4-[(1R)-1-aminopropyl]-6-methoxy-2-{6-[4-(propan-2-yl)-4H-1,2,4-triazol-3-yl]pyridin-2-yl}-2,3-dihydro-1H-isoindol-1-one 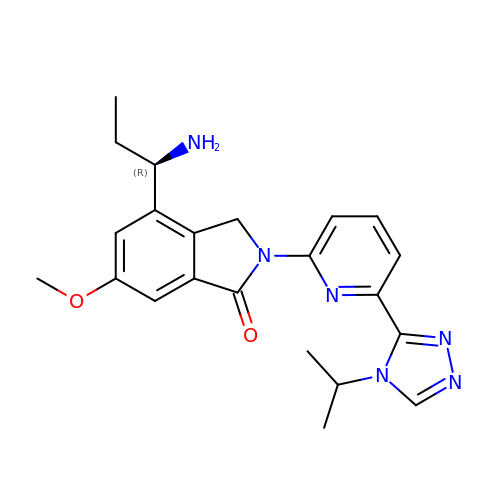| C22 H26 N6 O2 | RZQJOYYOKXRGDK-GOSISDBHSA-N> SCTRSIPPQ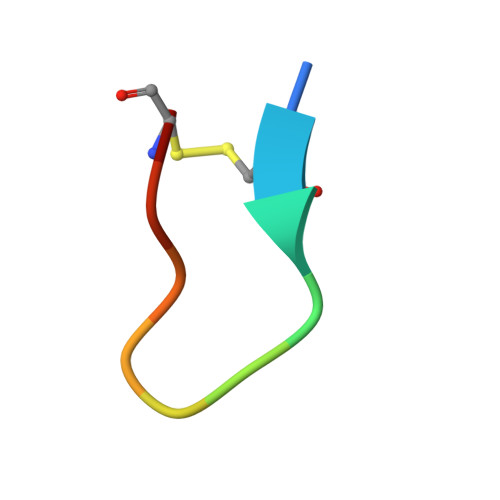CY(3R,4S)-1-[(4-amino-5H-pyrrolo[3,2-d]pyrimidin-7-yl)methyl]-4-{[(pent-4-yn-1-yl)sulfanyl]methyl}pyrrolidin-3-ol 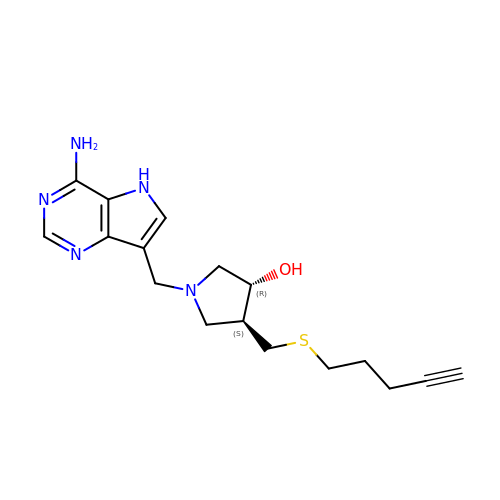| C17 H23 N5 O S | QRFSYYUFBJRRLL-KGLIPLIRSA-N> LNWKQDSNPLYKSAITTTINPR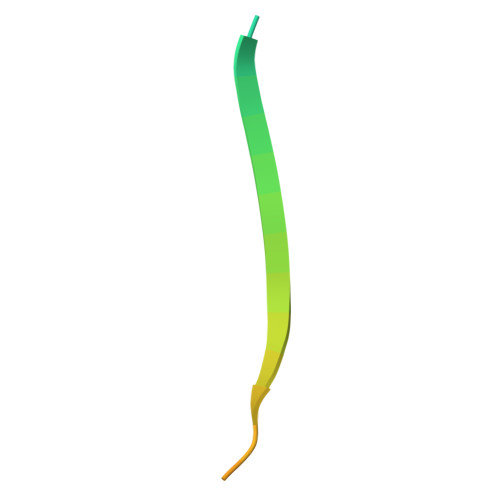FQEADSPTL> TNVISTLDLNLLTKGGGSWNVDGVNMKKSAVTTFDGKRVVKAVYDKNSGTSANPGVGGFSFSAVPDGLNKNAITFAWEVFYPKGFDFARGGKHGGTFIGHGAASGYQHSKTGASNRIMWQEKGGVIDYIYPPSDLKQKIPGLDPEGHGIG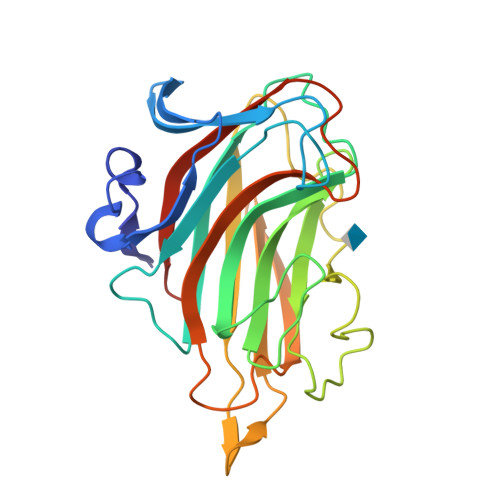FFQDDFKNALKYDVWNRIEIGTKMNTFKNGIPQLDGESYVIVNGKKEVLKRINWSRSPDLLISRFDWNTFFGGPLPSPKNQVAYFTNFQMKKYELEHHHHHH1-((1R)-1-(HYDROXYMETHYL)-3-{6-[(5-PHENYLPENTANOYL)AMINO]-1H-INDOL-1-YL}PROPYL)-1H-IMIDAZOLE-4-CARBOXAMIDE 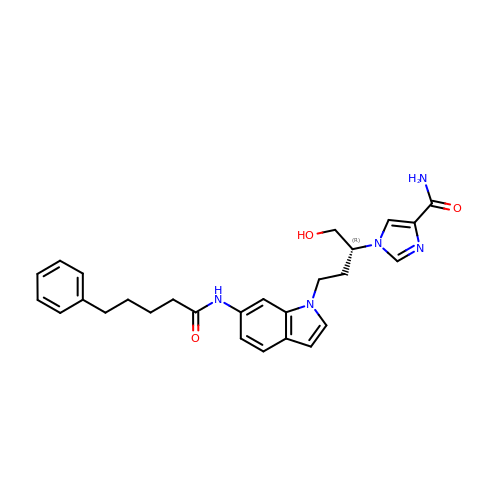| C27 H31 N5 O3 | SLLHIZOLSGWMLR-HSZRJFAPSA-N>[2x]QDYGGSQPEAY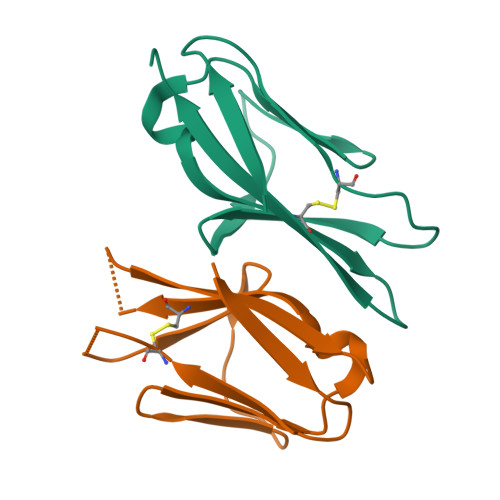VVAPGESLELQCMLKDAAVISWTKDGVHLGPNNRTVLIGEYLQIKGATPRDSGLYACTAARTVDSETWIFMVNVTDAAENLYFQ> MPFPFGKSHKSPADIVKNLKESMAVLEKQDISDKKAEKATEEVSKNLVAMKEILYGTNEKEPQTEAVAQLAQELYNSGLLSTLVADLQLIDFEGKKDVAQIFNNILRRQIGTRTPTVEYICTQQNILFMLLKGYESPEIALNCGIMLRECIRHEPLAKIILWSEQFYDFFRYVEMSTFDIASDAFATFKDLLTRHKLLSAEFLEQHYDRFFSEYEKLLHSENYVTKRQSLKLLGELLLDRHNFTIMTKYISKPENLKLMMNLLRDKSRNIQFEAFHVFKVFVANPNKTQPILDILLKNQAKLIEFLSKFQNDRTEDEQFNDEKTYLVKQIRDLKRPAQQEAGSGATNFSLLKQAGDVEENPG;> PHHHHHHENLYFQGMSFLTNDASSESIASFSKQEVMSSFLPEGGCYELLTVIGKGFEDLMTVNLARYKPTGEYVTVRRINLEACSNEMVTFLQGELHVSKLFNHPNIVPYRATFIADNELWVVTSFMAYGSAKDLICTHFMDGMNELAIAYILQGVLKALDYIHHMGYVHRSVKASHILISVDGKVYLSGLRSNLSMISHGQRQRVVHDFPKYSVKVLPWLSPEVLQQNLQGYDAKSDIYSVGITACELANGHVPFKDMPATQMLLEKLNGTVPCLLDTSTIPAEELTMSPSRSVANSGLSDSLTTSTPRPSNGDSPSHPYHRTFSPHFHHFVEQCLQRNPDARPSASTLLNHSFFKQIKRRASEALPELLRPVTPITNFEGSQSQDHSGIFGLVTNLEELEVDDWEFGSGATNFSLLKQAGDVEENPG;> PDYKDDDDKENLYFQGMEVVDPQQLGMFTEGELMSVGMDTFIHRIDSTEVIYQPRRKRAKLIGKYLMGDLLGEGSYGKVKEVLDSETLCRRAVKILKKKKLRRIPNGEANVKKEIQLLRRLRHKNVIQLVDVLYNEEKQKMYMVMEYCVCGMQEMLDSVPEKRFPVCQAHGYFCQLIDGLEYLHSQGIVHKDIKPGNLLLTTGGTLKISDLGVAEALHPFAADDTCRTSQGSPAFQPPEIANGLDTFSGFKVDIWSAGVTLYNITTGLYPFEGDNIYKLFENIGKGSYAIPGDCGPPLSDLLKGMLEYEPAKRFSIRQIRQHSWFRKKHPPAEAPVPIPPSPDTKDRWRSMTVVPYLEDLHGADEDEDLFDIEDDIIYTQDFTVPGQVPEEEASHNGQRRGLPKAVCMNGTEAAQLSTKSRAEGRAPNPARKACSASSKIRRLSACKQQ

In this study, we evaluated the Gatan Alpine detector, designed for operation at 100 and 200 keV. In addition to collections with a standard apoferritin sample, we also tested the performance of the Gatan Alpine detector on the LKB1-STRADα-MO25α complex (referred to hereafter as the LKB1 complex), which is considerably smaller (115 kDa) and asymmetric. Additionally, we obtained 3.2 Å resolution reconstruction of a 115 kDa asymmetric LKB1-STRADα-MO25α protein complex collected using Gatan Alpine on a TFS Glacios at 120 keV, demonstrating the applicability of this detector to more challenging biological samples.

Notably, the LKB1 sample was resolved to a higher resolution at 120 keV than at 200 keV (~ 3.2 Å vs. ~ 3.4 Å, respectively), with the local resolution ranges and Q-score metrics following similar trends as the FSC resolutions. To compare Gatan Alpine’s performance to the best imaging setup available to us, we also imaged the LKB1 complex with a TFS Titan Krios G2 at 300 keV with a BioQuantum energy filter and a K3 camera. Again, we started with a comparable initial number of particles for image processing and reached a similar final particle stack size. This yielded a reconstruction at 2.86 Å which was the highest resolution reconstruction out of all LKB1 complex datasets. Overall, the global conformation is similar to the crystal structure even though no nucleotide was added during sample preparation and we observed an apo LKB1 and an ADP-bound STRADα. Additionally, we were able to build some previously unresolved flexible loops and also observed some missing regions of the heterotrimeric complex in comparison to the crystal structure. Specifically, no density was observed for the STRADα Trp-Glu-Phe motif within the MO25α hydrophobic pocket although it was present in the construct and has been previously observed in both of the crystal structures. This motif is known to be required for MO25α recognition and binding in the absence of LKB1. Another region not resolved in our structure as compared to the crystal structure was the C-terminus of STRADα (residues 401–414). This may be due to the fact that it packs against the next molecule in the asymmetric unit in the crystal, packing not available in single-particle cryo-EM. Additionally, we resolved a more complete LKB1 C-terminal flanking tail (residues 311–347) at the LKB1-STRADα interface, resulting in novel interactions with STRADα.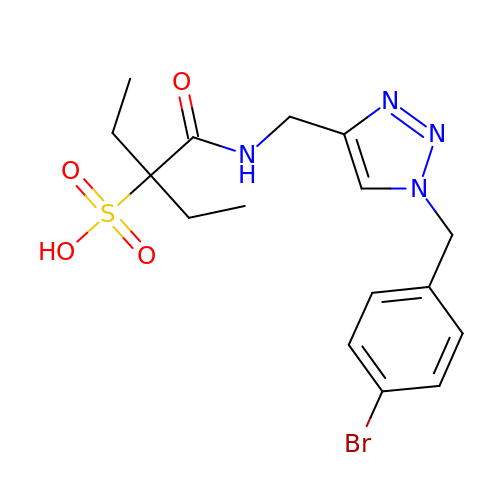3-[[1-[(4-bromophenyl)methyl]-1,2,3-triazol-4-yl]methylcarbamoyl]pentane-3-sulfonic acid | C16 H21 Br N4 O4 S | XOALJRIEKUWYNB-UHFFFAOYSA-N>RFYVKDHRNKAMINLHIQKDNPKIVHAFDMEDLGDKAVYCRCWRSKKFPFCDGAHTKHNEETGDNVGPL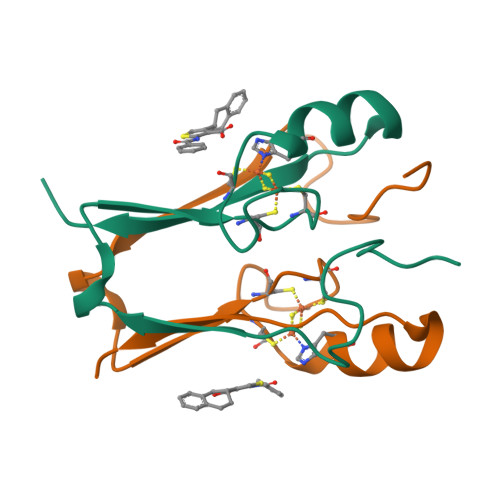IIKKKET[2x]> ITGTSTVGVGRGVLGDQKNINTTYSTYYYLQDNTRGNGIFTYDAKYR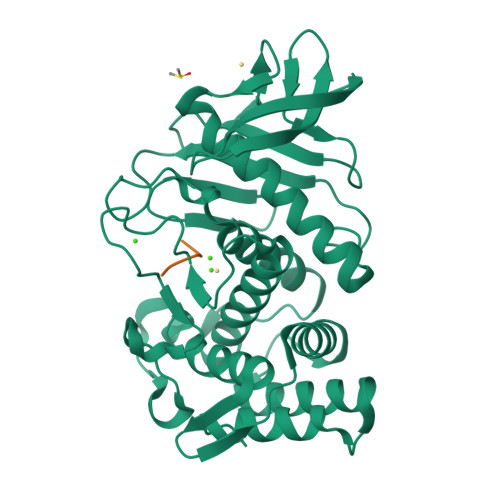TTLPGSLWADADNQFFASYDAPAVDAHYYAGVTYDYYKNVHNRLSYDGNNAAIRSSVHYSQGYNNAFWNGSQMVYGDGDGQTFIPLSGGIDVVAHELTHAVTDYTAGLIYQNESGAINEAISDIFGTLVEFYANKNPDWEIGEDVYTPGISGDSLRSMSDPAKYGDPDHYSKRYTGTQDNGGVHINSGIINKAAYLISQGGTHYGVSVVGIGRDKLGKIFYRALTQYLTPTSNFSQLRAAAVQSATDLYGSTSQEVASVKQAFDAVGVK;> GAIIG>MGSLCSKGQPVAQEEDEERERELTRQLKQEDRIEKNVYKLLLLGSGESGKSTIFKQIKLLYNTGFGVEELKNYTPVIHANVYQAIKILYEGCLDLQKKDVSGEYTMRRENMEHGKRIAEIGDGVDYHPIGLLESDLIAQIWSDPAIQATYRKANELQLPDCTEYFLSGVDRLAKPDYIPTEEDILHARVRTTGIADVVFKHDGHTYRVFDVGGQRNERRKWLHLFDGVKAVIFCAALSEYDQNLFEDEGKNRMVETMELFESVLRHPSFEKTSFLVFLNKYDIFRKKVLSVPLNVCEVFRDYNEVQGDQERKISHALQYIKNKFDEIYKRNTPGLGTQRLCWLFETTALDPRIMKYTFELVDKNLVVSSISLL[2x]

In all organisms, the core G-protein complex consists of one subunit each of the α, β, and γ proteins and exists in bimodal active versus inactive states. Signaling is initiated when the bound GDP is exchanged for GTP on Gα, which results in conformational changes that dissociate the heterotrimeric complex into Gα·GTP and Gβγ. To avoid response saturation by active Gα proteins, faster deactivation is achieved with the help of GTPase activity accelerating proteins (GAP), such as the regulator of G-protein signaling (RGS), which binds to activated Gα to accelerate GTP-hydrolysis. The two domains of the Gα—the Ras-like domain and the helical domain (HD)—flank the guanine nucleotide binding site.

To gain a broader perspective on the regulation of Gα in plants, we performed a structure-function analysis of Gα proteins from a lycophyte Selaginalla moellendorffi (SmGPA), a member of the earliest diverging group of modern vascular plants, and a monocot Oryza sativa (rice, OsRGA1), which does not have an RGS gene in its genome. The Ras-like GTPase domain of SmGPA with the GTP analog consists of five α-helices (α1, α9-12) surrounding a six-stranded β-sheet (β1a-b1f) with the helical domain (α2-α7) connected by two linking segments. In the SmGPA·GTPγS complex structure, the guanine nucleotide analog is bound in a highly conserved active site to provide a view of the active GTPase located between the Ras-like GTPase and the helical domains. The guanine ring of GTPγS is bound through interactions with Asn279, Lys280, Asp282, Ala384, and Leu349, and the ribose hydroxyl groups hydrogen bond with the backbone carbonyl of His186. In the active GTPase configuration of SmGPA, the three dynamic "switch" regions (switch I - Ala187-Val198; switch II - Val208-Ala230; switch III - Asp241-Arg252) involved in GTP binding and hydrolysis encompass the terminal group of bound GTPγS. In addition to the amine group of Lys50, Asp210 and Gln214 in switch II orient the terminal phosphate. Asp210 does this through interaction with the Mg2+ ion and Gln214 through hydrogen bonding with the γ-phosphate. Hydrogen bonding between the side-chain hydroxyl group of Thr191 and the γ-phosphate locks the switch I loop to bring Arg188 into position for the hydrolysis reaction. Beyond the active site, residues in switch III interact with residues in the helical domain to bring the two halves of SmGPA together. In the active GTPγS-bound structure, the conformation of the three switch regions favors interaction with the RGS protein, which is also confirmed by ITC analysis of the SmGPA:SmRGS interaction.> EDRLKIDVIDWLVFDPAQRAEALKQGNAIMRKFLASKKHEAAKEVFVKIPQDSIAEIYNQCEEQGMESPLPAEDDNAIREHLCIRAYLEAHETFNEW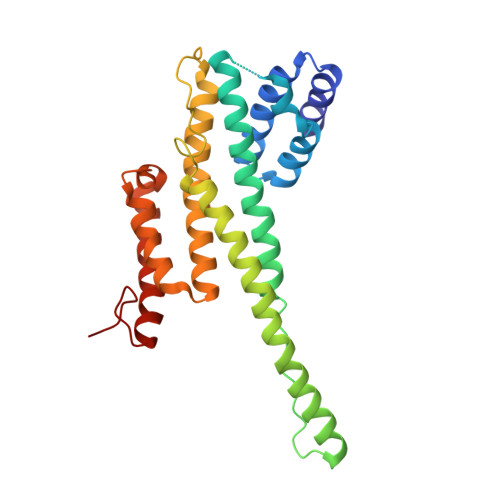FKHMNSVPQKPALIPQPTFTEKVAHEHKEKKYEMDFGIWKGHLDALTADVKEKMYNVLLFVDGGWMVDVREDAKEDHERTHQMVLLRKLCLPMLCFLLHTILHSTGQYQECLQLADMVSSERHKLYLVFSKEELRKLLQKLRESSLMLLDQGLDPLGYEIQ>GG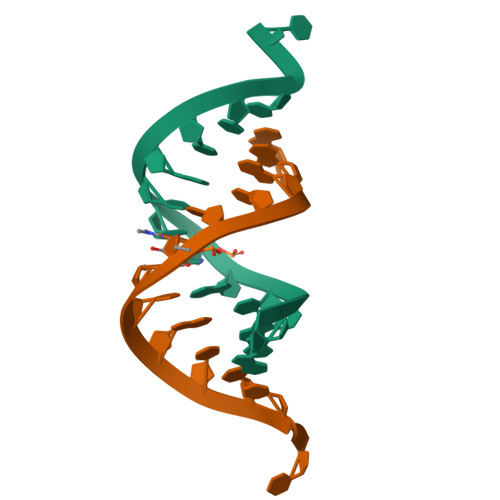ACGGACGUCCU[2x]Proper operation of the pivotal CME cargo adaptor AP2 requires membrane-localized Fer/Cip4 homology domain-only proteins (FCHO). The AP2 complex, composed of α, β2, μ2, and σ2 subunits, is pivotal to mammalian CCV formation, and its deletion is embryonically lethal in mice. FCHO1 and FCHO2 are similar in overall domain arrangement —folded N-terminal acidic phospholipid-binding homodimerization F-BAR domains and C-terminal folded μ-homology domains (μHD) separated by a ~300-residue, low-complexity intrinsically disordered protein linker, which has been suggested to participate in AP2 activation, although how it does so is undetermined. We dissect the network of interactions between the FCHO interdomain linker and AP2, which concentrates, orients, tethers, and partially destabilizes closed AP2 at the plasma membrane.

Since FCHO1 and FCHO2 have been suggested to bind the AP2 appendages, we investigated this possibility. No binding was observed between the different C blocks and the AP2 β2-appendage. Crystals of the α-appendage were grown in space group C2221 in the presence of a 10-fold molar excess of FCHO1 C peptide (residues 426 to 448, SEEQVSKNLFGPPLESAFDHEH), which diffracted to 1.4-Å resolution. Although the peptide bound to the top platform site of α-appendage in the same position as FXDXF and DP[FW] motifs, the orientation is opposite to that in these previously determined structures. The conserved hydrophobic interactions by the FCHO1 LFGPXL Phe436 and Leu440 (equivalent to FCHO2 residues 431 and 435) anchored the peptide to the α-appendage in the same positions as the phenylalanines of the FXDXF motif, facilitated, in part, by FCHO1 Pro438 being in a cis conformation: Mutations in FCHO1 FG to AA, LES to AAA, and PP to GG reduce binding to α-appendage to below detectable levels. H bonds between the LFGPXL motif’s main chain and α-appendage side chains further stabilize the interaction. (D) ITC showing ~50 μM KD binding of LFGPPL to α-appendage. Mutation of FG to SS, LES to AAA, and PP to SS all reduces binding to weaker than 500 μM KD. Thus, C blocks of all muniscin family members can bind to the α-appendage platform in a manner that is competitive with the binding of FxDxF and DP[FW] motifs of accessory CME proteins, and in addition, the partially overlapping WxxL sequence found only in FCHO2 can bind to the Cμ2 YxxΦ cargo–binding site and therefore potentially stabilize the unclosed but not-yet-open form of AP2.

> GSPGILAPLAPGSEDNFARFVCKNNGVLFENQLLQIGLKSEFRQNLGRMFIFYGNKTSTQFLNFTPTLICADDLQTNLNLQTKPVKPTVDGGAQVQQVVNIECISDFTEAPVLNIQFRYGGTFQNVSVKLPITLNKFFQPTEMASQDFFQRWKQLSNPQQEVQNIFKAKHPMDTEITKAKIIGFGSALLEEVDPNPANFVGAGIIHTKTTQIGCLLRLEPNLQAQMYRLTLRTSKDTVSQRLCELLSEQF;> QSEEQVSKNLFGPPLESAFDHED4-HYDROXY-ACONITATE ION | C6 H3 O7 | 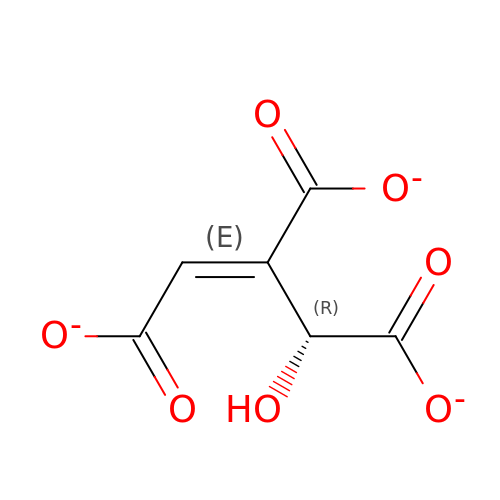WUUVSJBKHXDKBS-ROFOPDMZSA-K> SMTMINGYEQSDREEKIDILNLESLEKQAEEIIPAGGFGYIAGGSEDEWTLKQNRMAFHH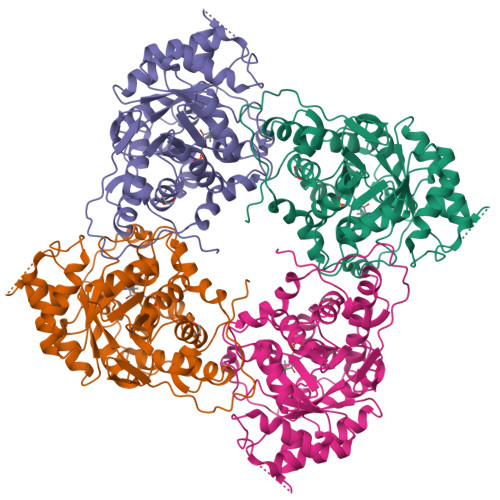RQIAPKALSGIEKPELNTEIFGIPLNTPVMMAPAAAQGLAHSQGEKDTARGLAAVGGLMAQSTYSSVSIAETAAAGGDAPQFFQLYMSKDWNFNESLLDEAKKANVKAIILTVDATVDGYREADIKNKFTFPLPMANLIKFSEGNGQGKGIEEIYASAAQNIRPEDVKRIADYTNLPVIVKGIQTPEDAIRAIDAGAAGIYVSNHGGRQLNGGPASFDVLEDIATAVNKQVPIIFDSGVRRGSDVFKALASGADLVALGRPVIYGLALGGAKGVQSVFEHLNHELEIVMQLAGTKTIEDVKNNSLLNIKY> GLPVCAETCVGGTCNTPG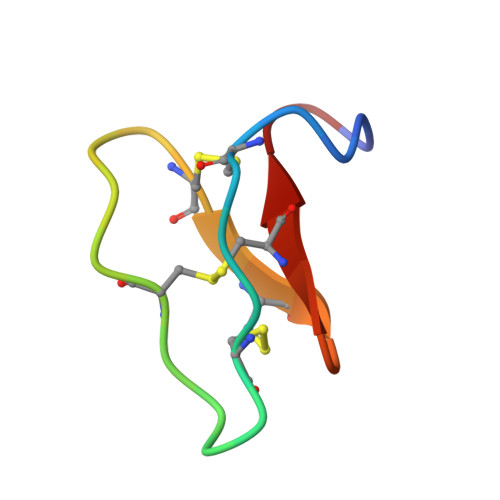CTCSWPVCTRN;> GLPVCGETCVGGTCNTPGCTCSWPVCTRN>[2x]MTSVHFNPGLDSKEVNGNSVKEEAEVQIGDGKEETKDPDTMYHQVRKKITPFVMSFGFRVFGLVLIILDIIMVIVDLSLSEKSRDVGGALETVSLVISFFFLIDVLLRVYVEGFKVYFSSKLNIVDACIVVITLVVTMIYAFSDFSGASLIPRV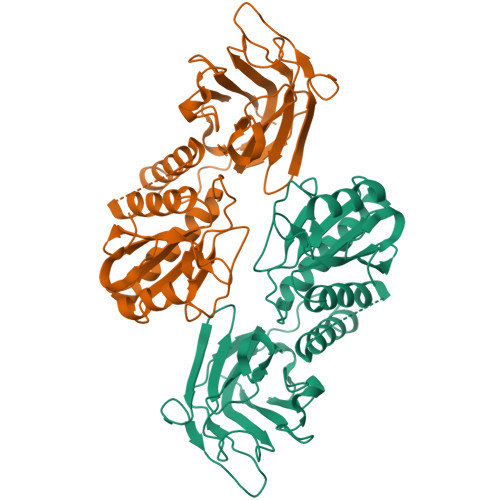VTFLRSLRILILVRIFRLASQKRELEKVTRRMVSENKRRYQKDGFDLDLTYVTERVIAMSFPSSGKQALYRNPIREVVRFLDTKHMDHYKVFNLCSEKGYDPKFFHYRVERVMIDDHNVPSLDDMLRYTACVRDWMAADSRNVIAIHSKGGKGRTGTMVCTWLIDSDQFESAQESLDYFGERRTDKSMSSKFQGVETPSQSRYVGYYEIMKNQYNRQLPPRKSLKIKSIRIHSIAGVGKGNGSDLKLKIIVKHELVFQCVCAKQHNCTVFPDTGSNAVVISLQDGPIVTGDVKVMFESSAGLPKGYEDCPFYFWFNTSFVENYRLFLSREELDNPHKPKTWDIYKEDFGVTLSFTEPSNSLEVLFQ>MPVLENRAAQGDITAPGGARRLTGDQTAALRDSLSDKPAKNIILLIGNGMGDSEITAARNYAEGAGGFFKGIDALPLTGQYTHYALNKKTGKPDYVTDSAASATAWSTGVKTYNGALGVDIHEKDHPTILEMAKAAGLATGNVSTAELQDATPAALVAHVTSRKCYGPSATSEKCPGNALEKGGKGSITEQLLNARADVTLGGGAKTFAETATAGEWQGKTL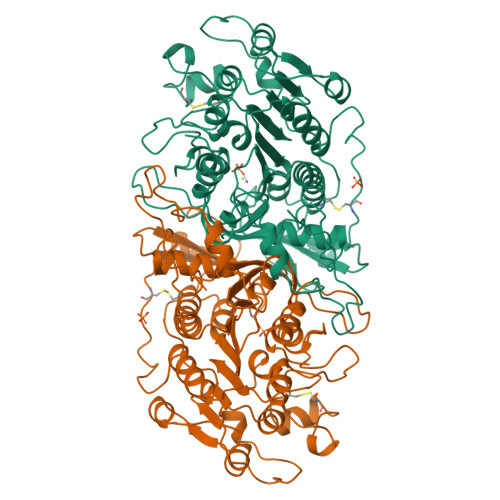REQAQARGYQLVSDAASLNSVTEANQQKPLLGLFADGNMPVRWLGPKATYHGNIDKPAVTCTPNPQRNDSVPTLAQMTDKAIELLSKNEKGFFLQVEGASIDKQDHAANPCGQIGETVDLDEAVQRALEFAKKEGNTLVIVTADHAHASQIVAPDTKAPGLTQALNTKDGAVMVMSYGNSEEDSQEHTGSQLRIAAYGPHAANVVGLTDQTDLFYTMKAALGLK[2x]2-cyclopropyl-~{N}-(4-iodophenyl)quinazolin-4-amine 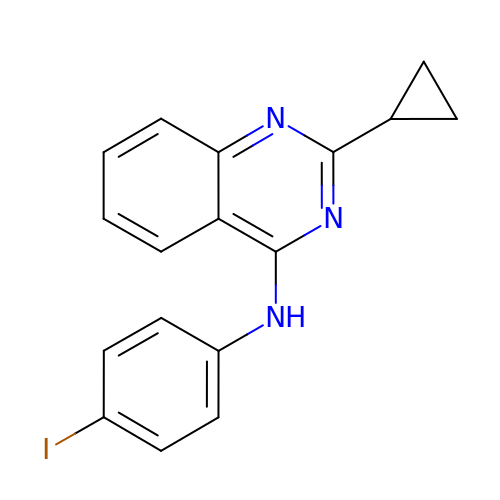| C17 H14 I N3 | JENOGSHDNMPWIS-UHFFFAOYSA-N> LSLKGKKLDFFGRGDTYVSLIDTIPELSRFTACIDLVFMDDNSRYWMAFSYITNNALLGREDIDLGLAGDHQQLILYRLGKTFSIRHHLASFQWHTICLIWDGVKGKLELFLNKERILEVTDQPHNLTPHGTLFLGHFLKNESSEVKSMMRSFPGSLYYFQLWDHILENEEFMKCLDGNIVSWEEDVWLVNKIIPTVDRTLRCFVPENMTIQEKSGGGGAGGGGGTDDDDKWSHPQFEK

Here, we showcase the example of ADGRG4, an orphan aGPCR that possesses a PTX-like domain at its very N-terminal tip, followed by an extremely long stalk containing serine-threonine repeats. Using X-ray crystallography and biophysical methods, we determined the structure of this unusual PTX-like domain and provide experimental evidence for a homodimer equilibrium of this domain which is Ca2+-independent and driven by intermolecular contacts that differ vastly from the known soluble PTXs. However, only three domains are predicted by homology within this huge ECR—the PTX-like domain, the hormone receptor binding motif (HRM), and the GPCR autoproteolysis-inducing (GAIN) domain. Our data alongside of theoretical considerations lead to the hypothesis that ADGRG4 acts as an in vivo sensor for shear forces in enterochromaffin and Paneth cells of the small intestine.

The crystallographic data revealed a β-sandwich fold. Six and seven antiparallel β-strands assemble the two β-sheets A and B, respectively. The A face is covered by another loop of residues 189 to 205 with a short helical stretch. This loop coordinates a metal ion via the side chain carboxy group of the residue D202. Two disulfide bridges stabilize the protein fold. C58-C123 links strands β3 and β8 in the β-sheet of the A face. C200-C228 connects the long A face loop 189-205 with the C-terminal residues of the PTX-like domain. The unit cell of the G4-PTX crystals on the other hand contained only a single protein chain in the asymmetric unit. However, there is only one interface generated by point symmetry that exhibits a sufficient surface area for homodimerization. Two protomers interact such that the two strands at the edge of the sandwiched β-sheet interact with those of the other molecule (β7 with β10′ and β10 with β7′).> PKHGKRYRALLEKVDPNKIYTIDEAAHLVKELATAKFDETVEVHAKLGIDPRRSDQNV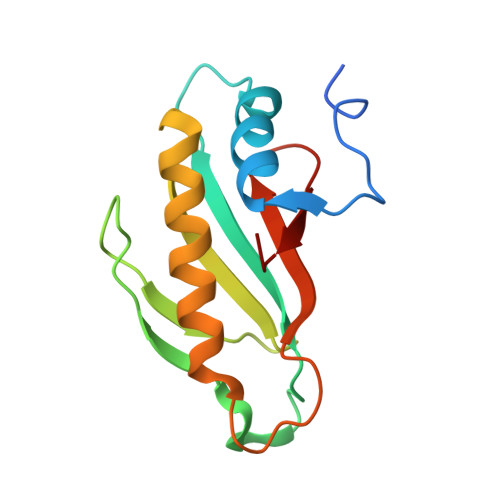RGTVSLPHGGRIEFRNDKTGAIHAPVGKASFPPEKLADNIRAFIRALEAHKPEGAKGTFLRSVYVTTTMGPSVRINPHS>MSAAAEVLARNQELLTAIAAGNYEKYATMCDPSMTCFEPEAVGHLVEGLDFHKYYFTMPSAPPAPDAPKPHVLNTMASPHVRMVGDSCAVVSYIRLTQKMVNGAPVTVQAEETRVWEKKDGGWIHVHMHRSLVK[9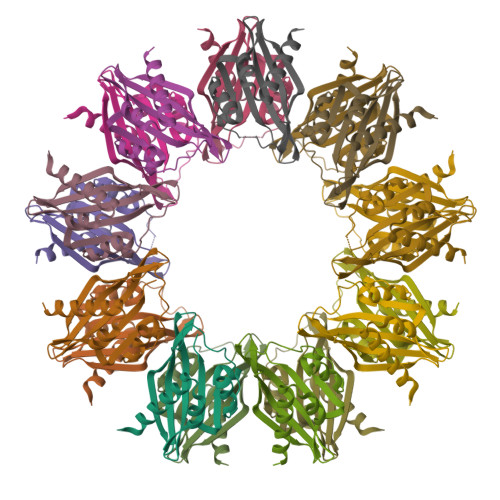x]>HHHHHHASENLYFQGAMASEKHFKYVILGGGVAAGYAAREFAKQGVKPGELAIISKEAVAPYERPALSKGYLFPQNAARLPGFHVCVGSGGERLLPEWYSEKGIELILSTEIVKADLASKTLTSAVGATFTYEILIIATGSSVIKLSDFGTQGADSNNILYLREVDDADKLVAAIQAKKGGKAVIVGGGYIGLELSAALKINDFDVTMVFPAPWCMPRLFTADIAAFYESYYTNKGVKIVKGTVAVGFDADANGDVTAVNLKNGSVLEADIVVVGVGGRPLTTLFKGQVAEEKGGIKTDAFFETSVPGVYAVGDVATFPMKMYNELRRVEHVDHARKSAEQAVKAIKGKESGESVVEYDYLPYFYSRSFDLGWQFYGDNVGDTILFGDSDPTSAKPKFGSYWIKDGKVLGAFLEGGSPDENKAIAKVAKTQPPVANIEELKKEGLQFASKI[2x]

MDHAR reduces the monodehydroascorbate (MDHA) radical to AsA at the expense of an NAD(P)H molecule, with NADH being the preferred donor. We report, for the first time, the crystal structure of MDHAR of O. sativa L. japonica (OsMDHAR) to understand its detailed mechanism. Structural comparison of OsMDHAR to other proteins, using the DALI server, indicated that it has the same fold as that of putidaredoxin reductase (Pdr), biphenyl dioxygenase (BphA4)18 and rubredoxin reductase (RdxR). All these proteins consist of three domains: an NAD(P)-binding domain, an FAD-binding domain, and a C-terminal domain, as shown in Figs 1 and 2.

For more detailed information, we attempted to determine the structure of the enzyme in complex with NADP. We prepared an E196A mutant protein, which facilitates the binding of NADP by eliminating the carboxylic acid group. Unexpectedly, the structure of the E196A mutant-NADP complex revealed that the 2′-phosphate group of NADP was not located in the position of the carboxylic acid group of Glu196. ITC experiments clearly showed an increase in the affinity of OsMDHAR toward NADP on removing the carboxylate group of Glu196. Although there is no difference between WT and E196A in NAD binding affinity, E196A showed a 16-fold increase in affinity for NADP compared to the WT. Therefore, together from the structural studies and ITC experiments, we hypothesized that Glu196 has an important role in the NAD selectivity of the OsMDHAR.5-(1-methyl-4,5-dihydro-1H-pyrrol-2-yl)pyridin-2-ol | 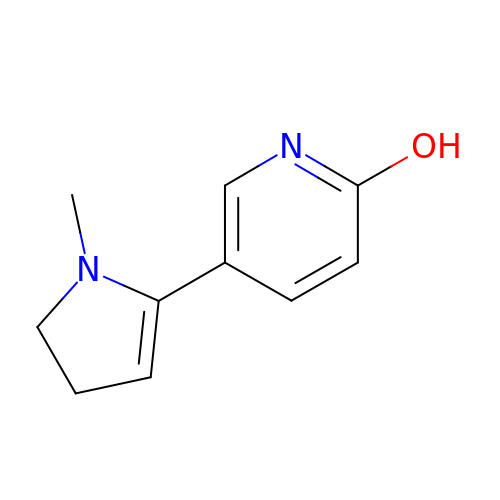C10 H12 N2 O | LWGKCPAYDQWMMS-UHFFFAOYSA-N>[8x]MSDKDSKNTPQVPEKLGLSRRGFLGASAVTGAAVAATALGGAVMTRESWAQAVKESKQKIHVGPGELDDYYGFWSGGHQGEVRVLGVPSMRELMRIPVFNVDSATGW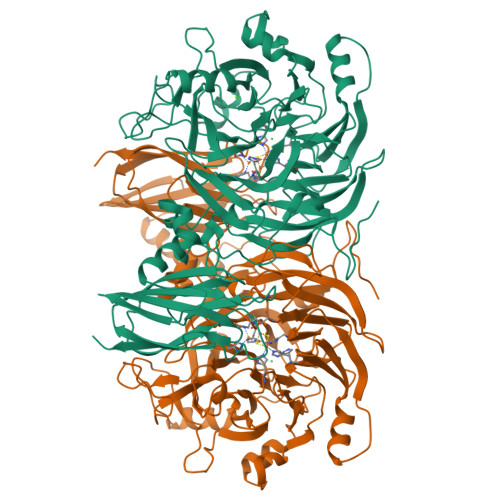GLTNESRHIMGDSAKFLNGDCHHPHISMTDGKYDGKYLFINDKANSRVARIRLDIMKCDKMITVPNVQAIHGLRLQKVPHTKYVFANAEFIIPHPNDGKVFDLQDENSYTMYNAIDAETMEMAFQVIVDGNLDNTDADYTGRFAAATCYNSEKAFDLGGMMRNERDWVVVFDIHAVEAAVKAGDFITLGDSKTPVLDGRKKDGKDSKFTRYVPVPKNPHGCNTSSDGKYFIAAGKLSPTCSMIAIDKLPDLFAGKLADPRDVIVGEPELGLGPLHTTFDGRGNAYTTLFIDSQVVKWNMEEAVRAYKGEKVNYIKQKLDVHYQPGHLHASLCETNEADGKWLVALSKFSKDRFLPVGPLHPENDQLIDISGDEMKLVHDGPTFAEPHDCIMARRDQIKTKKIWDRNDPFFAPTVEMAKKDGINLDTDNKVIRDGNKVRVYMTSMAPAFGVQEFTVKQGDEVTVTITNIDQIEDVSHGFVVVNHGVSMEISPQQTSSITFVADKPGLHWYYCSWFCHALHMEMVGRMMVEPA> IPTTENLYFQGAMALEEIKNGTDISTLDIRKFNLNINNVSVLSKSQSVDQFHLSNPHYEYLSGGAYPGEMENFTLKVDKSKKQDQVFENPLSLKFTNIGTVNGKQVDAYLNFNKVTLHYLNTAQAESEMNSAQKSTVEFFSISELWESNAFEIGNVPYVDANHDYIMNKAFWIDADVTAEIRYADGTETDLKLVMKPTDIDAIDANNLKETFYVKNYQNDVNLRLMNNANVLVQEEASDRTSWIATQITGGSYNENNVSGLALRSNSNSMNFGYSSTETCSAVFGLYI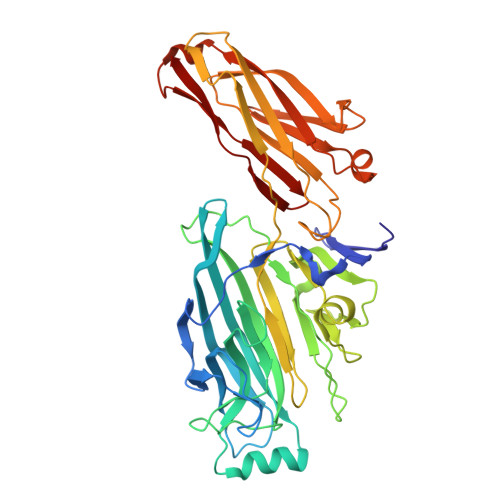EKIDPRPVLEVDPAEIPAKDGQDVTYKATFKVPVPGKDILAAPSSIEMVQKFDERLDYKELKVESGGVTLQEGRDYTIEKTGQTVTVKMTPEYLKGNSSSDIIITYKTATNKKVEEKGSEKIDNTVTLHVDNLSAPSNQVSTALLYEK>MNTDVRIEKDFLGEKEIPKDAYYGVQTIRATENFPITGYRIHPELIKSLGIVKKSAALANMEVGLLDKEVGQYIVKAADEVIEGKWNDQFIVDPIQGGAGTSINMNANEVIANRALELMGEEKGNYSKISPNSHVNMSQSTNDAFPTATHIAVLSLLNQLIETTKYMQQEFMKKADEFAGVIKMGRTHLQDAVPILLGQEFEAYARVIARDIERIANTRNNLYDINMGATAVGTGLNADPEYISIVTEHLAKFSGHPLRSAQHLVDATQNTDCYTEVSSALKVCMINMSKIANDLRLMASGPRAGLSEIVLPARQPGSSIMPGKVNPVMPEVMNQVAFQVFGNDLTITSASEAGQFELNVMEPVLFFNLIQSISIMTNVFKSFTENCLKGIKANEERMKEYVEKSIGIITAINPHVGYETAAKLAR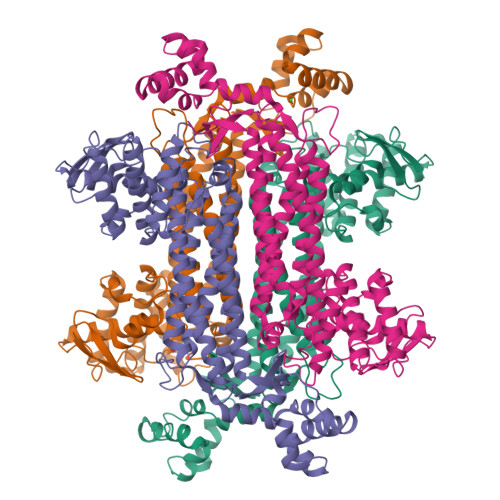EAYLTGESIRELCIKYGVLTEEQLNEILNPYEMIHPGIAGRK[8x]>VQEAQANTESEKRRLDSVITHMSDGIIATDRRGRIRIVNDMALKMLGMAKEDIIGYYMLSVLSLEDEFKLEEIQENNDSFLLDLNEEEGLIARVNFSTIVQETGFVTGYIAVLHDVTEQQVVERER[2x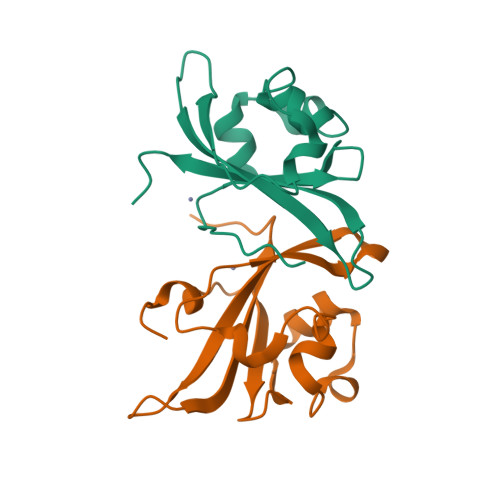]>GPGTMMNVIMREIGKKLDELSREFY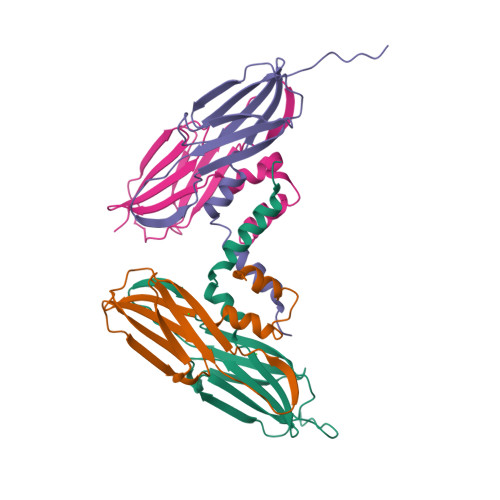ESVIPPIDMYEEGGELVVVADLAGFNKDKISVRLSAQNELIINAEREIQYIGTKYATQRPLKIHKVIRLPVKVKRDSQVTDKYENGVLTIRIPVEGSVSIRIE[4x]>GSHMVRESSFVEKMKKTGRNIIVFYGSQTGTAEEFANRLSKDAHRYGMRGMSADPEEYDLADLSSLPEIDNALVVFCMATYGEGDPTDNAQDFYDWLQETDVDLSGVKFAVFGLGNKTYEHFNAMGKYVDKRLEQLGAQRIFELGLGDDDGNLEEDFITWREQFWPAVCEHFGVEATGEESSIRQYELVVHTDIDAAKVYMGEMGRLKSYEN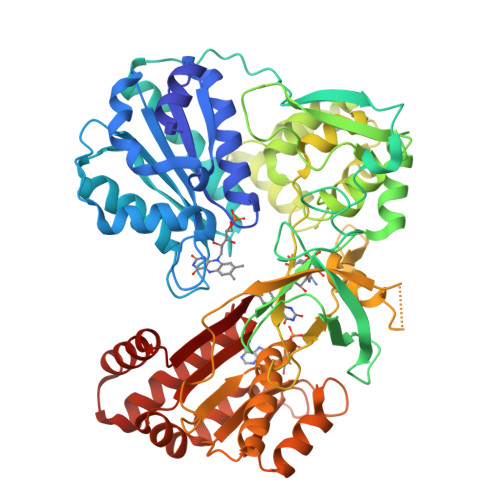QKPPFDAKNPFLAAVTTNRKLNQGTERHLMHLELDISDSKIRYESGDHVAVYPANDSALVNQLGKILGADLDVVMSLNNLDEESNKKHPFPCPTSYRTALTYYLDITNPPRTNVLYELAQYASEPSEQELLRKMASSSGEGKELYLSWVVEARRHILAILQDCPSLRPPIDHLCELLPRLQARYYSIASSSKVHPNSVHICAVVVEYETKAGRINKGVATNWLRAKEPAGENGGRALVPMFVRKSQFRLPFKATTPVIMVGPGTGVAPFIGFIQERAWLRQQGKEVGETLLYYGCRRSDEDYLYREELAQFHRDGALTQLNVAFSREQSHKVYVQHLLKQDREHLWKLIEGGAHIYVCGDARNMARDVQNTFYDIVAELGAMEHAQAVDYIKKLMTKGRYSLDVWS[2x]> MAVPFVEDWDLVQTLGEGAYGEVQLAVNRVTEEAVAVKIVDMK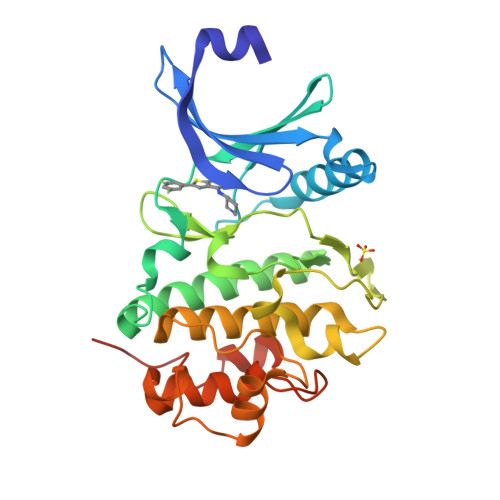RAVDCPENIKKEICINKMLNHENVVKFYGHRREGNIQYLFLEYCSGGELFDRIEPDIGMPEPDAQRFFHQLMAGVVYLHGIGITHRDIKPENLLLDERDNLKISDFGLATVFRYNNRERLLNKMCGTLPYVAPELLKRREFHAEPVDVWSCGIVLTAMLAGELPWDQPSDSCQEYSDWKEKKTYLNPWKKIDSAPLALLHKILVENPSARITIPDIKKDRWYNKPLKKGAKRP> GPGSTKQVPTEINPKFKDLRAYYTKPSLEFKNEIGIILKKWTTIRFMNVVPDYFIYKIALVGKDDKKYGEGVHRNVDVFVVLEENNYNLEKYSVGGITKSNSKKVDHKAGVRITKEDNKGTISHDVSEFKITKEQISLKELDFKLRKQLIEKNNLYGNVGSGKIVIKMKNGGKY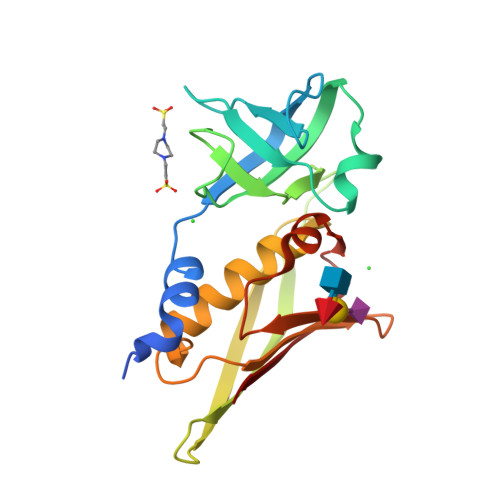TFELHKKLQENRMADVIDGTNIDNIEVNIK> MSIEIKTNSVEPIRHTYGHIARRFGDKPATRYQEASYDIEAKTNFHYRPQWDSEHTLNDPTRTAIRMEDWCAVSDPRQFYYGAYVGNRAKMQESAETSFGFCEKRNLLT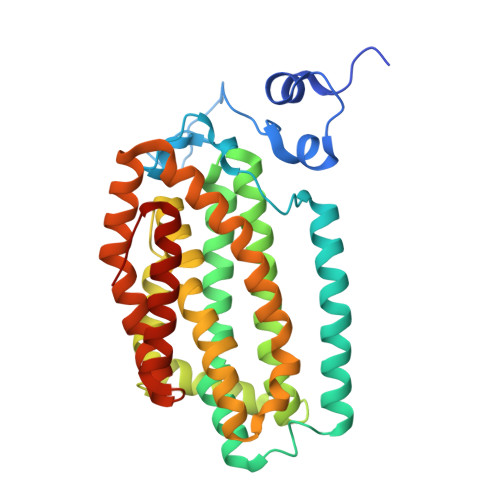RLSEETQKQLLRLLVPLRHVELGANMNNAKIAGDATATTVSQMHIYTGMDRLGIGQYLSRIALMIDGSTGAALDESKAYWMDDEMWQPMRKLVEDTLVVDDWFELTLVQNILIDGMMYPLVYDKMDQWFESQGAEDVSMLTEFMRDWYKESLRWTNAMMKAVAGESETNRELLQKWIDHWEPQAYEALKPLAEASVGIDGLNEARAELSARLKKFELQSRGVSA> SHSTAETTLDSFFSRAGLVGEIDLPLEGTTNPNGYANWDIDITGYAQMRRKVELFTYMRFDAEFTFVACTPTGQVVPQLLQYMFVPPGAPKPDSRESLAWQTATNPSVFVKLSDPPAQVSVPFMSPASAYQWFY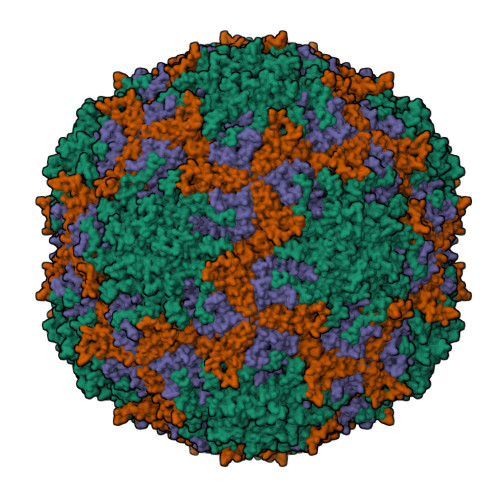DGYPTFGEHKQEKDLEYGACPNNMMGTFSVRTVGTSKSKYPLVIRIYMRMKHVRAWIPRPMRNQNYLFKANPNYAGNFIKPTGASRTAITT;> LTIGNSTITTQEAANIIVGYGEWPSYCSDSDATAVDKPTRPDVSVNRFYTLDTKLWEKSSKGWYWKFPDVLTETGVFGQNAQFHYLYRSGFCIHVQCNASKFHQGALLVAVLPEYVIGTVAGGTGTEDSHPPYKQTQPGADGFELQHPYVLDAGIPISQLTVCPHQWINLRTNNCATIIVPYINALPFDSALNHCNFGLLVVPISPLDYDQGATPVIPITITLAPMCSEFAGLRQ;> GFPTELKPGTNQFLTTDDGVSAPILPNFHPTPCIHIPGEVRNLLELCQVETILEVNNVPTNATSLMERLRFPVSAQAGKGELCAVFRADPGRSGPWQSTLLGQLCGYYTQWSGSLEVTFMFTGSFMATGKMLIAYTPPGGPLPKDRATAMLGTHVIWDFGLQSSVTLVIPWISNTHYRAHARDGVFDYYTTGLVSIWYQTNYVVPIGAPNTAYIIALAAAQKNFTMQLCKDASDIL>[2x]GHMRLLSEDLFKQSPKLSEQELDELANNLADYLFQAADIDWHQVISEKTRGLTTEEMAKSEHRYVQAFCR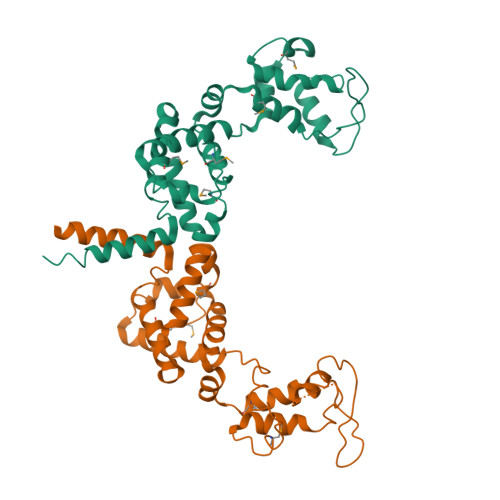EILKYPDCYKSADVASPESPKSGGGSVIDVALKRLQTGRERLFTTTDEKGNRELKKGDAILESAINAARMAISTEEKNTILSNNVKSATFEVFCELPCMDGFAEQNGKTAFYALRAGFYSAFKNTDTAKQDITKFMKDNLQAGFSGYSYQGLTNRVAQLEAQLAALSAKLS>DIWPSGGQMTVKDLTAKYTEGGNAILENISFSISPGQRVGLLGRTGSGKSTLLLAFLRLLNTEGEIQIDGVSWDSITLEQWRKA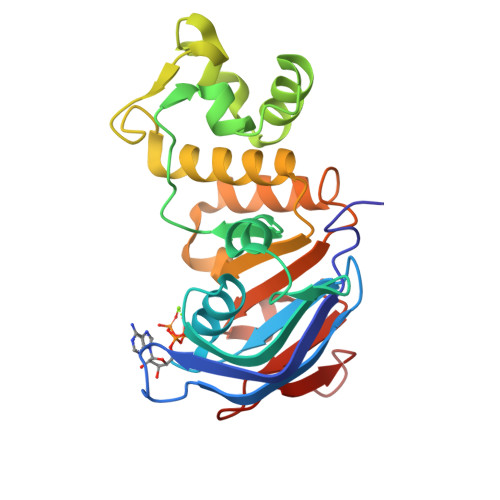FGVIPQDVFIFSGTFRKNLDPNEQWSDQEIWKVADEVGLRSVIEQFPGGLDFVLVDGGCVLSHGHKQLMCLARAVLSKAKILLLDEPSAHLDPVTYQIIRRTLKQAFADCTVILCEARIEAMLECDQFLVIEENKVRQYDSIQKL[4x]>TKKESFEDVLPSILNTITTNSELTEVPEVANWLKKVLEYNLAGGKKARGLTTLFAYEMLEKPENITEETIYLAKTLGWCVEILQGFLVMLDDIMDGSTTRRGVPCWYQLPEVGLAAVNDSSLMFSSIFYVLHAHFADKKIYTNLVELFNESLMHTSIGQHLDVTMERRQKSDYSLFTIERYNAIVKYKTAYYTYQLPVCLGMLLANISDPVLHQKAEDMCLEIGKFFQIQDDYIDCYGDESLTGKMGTDIQEAKCSWLAVMALQRCSASQKIVFTTCY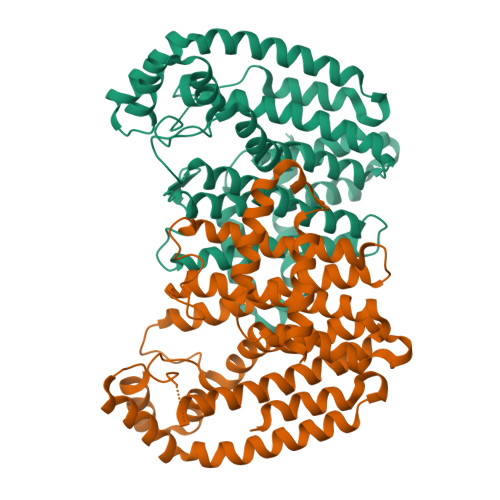GSKEPAHIERIKELYKQLQLPELYAQEETRMYESLIKQAHGLPSELSPALFVRLIHMIYKRNH[2x]> MGDTDKEYISEEVQKAIDDSVKQVFGIKDDSSQVTITYNKDKVNLWTQQIIDYTIRGLNKLGKHFKYCVTAILQQT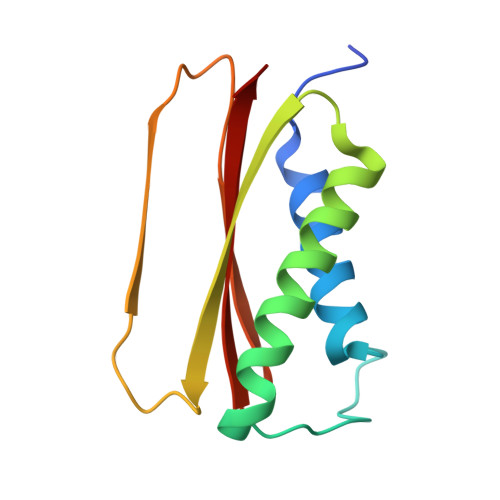NHAGISVQITAYQDTNTDGSLIQCYEINDIYAIVSVFAMAV4-methyl-~{N}-[(~{E})-oct-5-enyl]piperidine-1-carboxamide | C15 H30 N2 O | 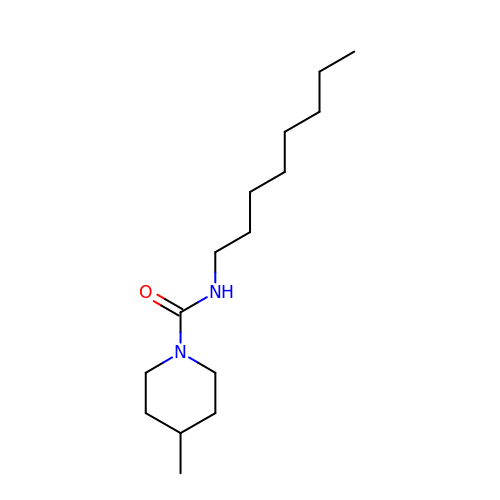HAWIGYZAJFCXMR-UHFFFAOYSA-N> MEAVIKVISSACKTYCGKTSPSKKEIGAMLSLLQKEGLLMSPSDLYSPGSWDPITAALSQRAMILGKSGELKTWGLVLGALKAAREEQVTSEQAKFWLGLGGGRVSP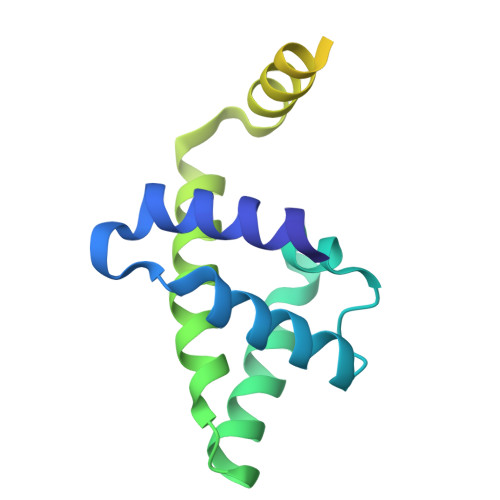PGPECIEKPATERRIDKGEEVGETTVQRDAKMAPEETATPKTVGTSCYRSHHHHHH The sole target for neutralizing antibodies on the virus surface is the envelope (Env) protein, a homotrimer consisting of three copies of gp120 and gp41 subunits that are associated by non-covalent interactions. Methods enabling the production of stable recombinant trimer immunogens based on the ectodomain of Env have catalyzed recent HIV vaccine efforts. Hence, the efficient trafficking of Env trimer immunogens to follicles following immunization is likely essential to promote optimal humoral responses to HIV. Here, we demonstrate two strategies to concentrate HIV Env immunogens in follicles, via the formation of immune complexes (ICs) or by employing self-assembling protein nanoparticles for multivalent display of Env antigens.

We employed a tetrahedral nanoparticle, T33_dn2, which consists of two trimeric building blocks (four copies of each), and can present four SOSIP trimers. For particle production, BG505 SOSIP-T33_dn2A was combined with equimolar amounts of the assembly component (T33_dn2B) and incubated for 24 h, leading to >90% assembly efficiency. An initial cryo-EM reconstruction of the entire nanoparticle verified the appropriate assembly to the target tetrahedral architecture with four BG505 SOSIP trimers flexibly linked to the nanoparticle core. The particle diameter is ~37 nm and the average apex–apex distance between the BG505 SOSIP trimers is 31 nm. Due to the flexible nature of the linker connecting the BG505 SOSIP antigen and T33_dn2A scaffold, high-resolution reconstruction of the entire nanoparticle as a single model could not be performed. However, focused refinement in combination with partial signal subtraction allowed us to treat the nanoparticle core (consisting of T33_dn2A and T33_dn2B) and the displayed BG505 SOSIP trimers as separate subparticles and analyze them independently. Using the approach described in the “Methods” section and Supplementary Fig. 3a, we reconstructed a 4.6 Å resolution map of the nanoparticle core and a 4.5 Å resolution map of the BG505 SOSIP trimer. The refined model of the T33_dn2 nanoparticle core revealed a high degree of correlation with the design model predicted by Rosetta at the backbone level. When compared to Rosetta models, Cα root-mean-square deviation values for the trimeric T33_dn2A and T33_dn2B components were 1.20 and 0.81 Å, respectively. The C-terminal helix in T33_dn2B was not resolved in the EM map, suggesting a high degree of flexibility, which may be at least partially influenced by the 6xHis-tag immediately following this sequence.

>GSMGNLAEKMYKAGNAMYRKGQYTIAIIAYTLALLKDPNNAEAWYNLGNAAYKKGEYDEAIEAYQKALELDPNNAEAWYNLGNAYYKQGDYDEAIEYYKKALRLDPRNVDAIENLIEAEEKQGAS[12x];>MEEAELAYLLGELAYKLGEYRIAIRAYRIALKRDPNNAEAWYNLGNAYYKQGDYREAIRYYLRALKLDPENAEAWYNLGNALYKQGKYDLAIIAYQAALEEDPNNAEAKQNLGNAKQKQGLEHHHHHH[12x]> MRWYPWLRPDFEKLVASYQAGRGHHALLIQALPGMGDDALIYALSRYLLCQQPQGHKSCGHCRGCQLMQAGTHPDYYTLAPEKGKNTLGVDAVREVTEKLNEHARLGGAKVVWVTDAALLTDAAANALLKTLEEPPAETWFFLATREPERLLATLRSRCRLHYLAPPPEQYAVTWLSREVTMSQDALLAALRLSAGSPGAALALFQGDNWQARETLCQALAYSVPSGDWYSLLAALNHEQAPARLHWLATLLMDALKRHHGAAQVTNVDVPGLVA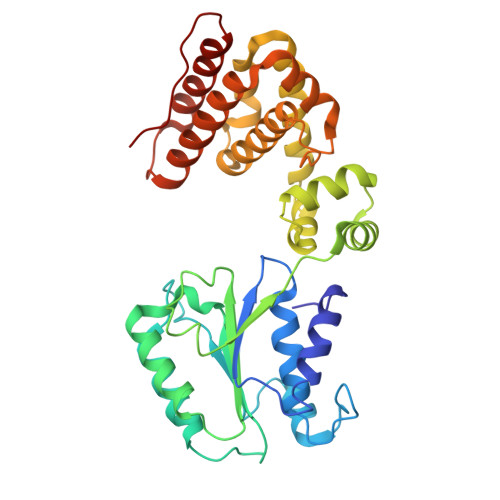ELANHLSPSRLQAILGDVCHIREQLMSVTGINRELLITDLLLRIEHYLQPGVVLPVPHL> GSHMSGWRLLLTRPDEECAALAASLGEAGVHSSSLPLLAIDPLEETPEQRTLMLDLDRYCA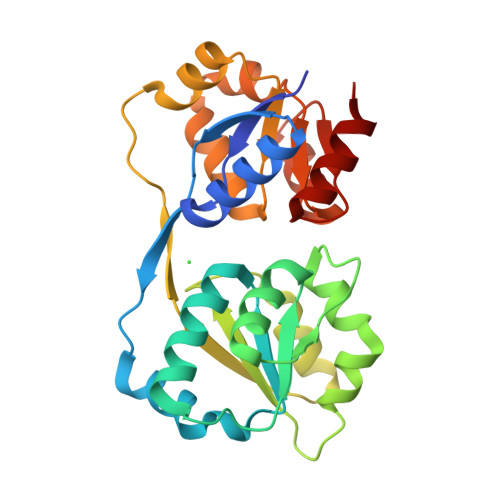VVVVSKPAARLGLERLDRYWPQPPQQTWCSVGAATAAILEAYGLDVTYPEQGDDSEALLALPAFQDSLRVHDPKVLIMRGEGGREFLAERLRGQGVQVDYLPLYRRRAPDYPAGELLARVRAERLNGLVVSSGQGLQNLYQLAAADWPEIGRLPLFVPSPRVAEMARELGAQRVIDCRGASAPALLAALTSAA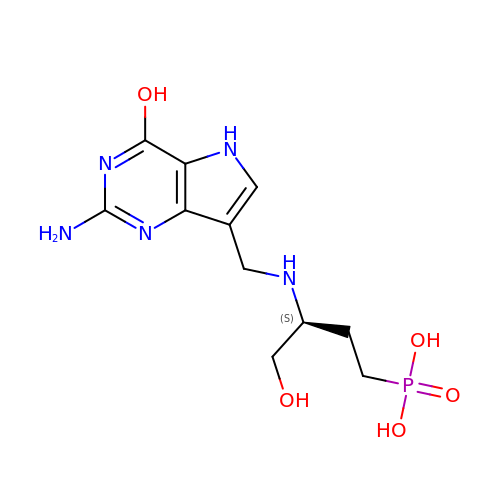[(3S)-3-{[(2-amino-4-hydroxy-5H-pyrrolo[3,2-d]pyrimidin-7-yl)methyl]amino}-4-hydroxybutyl]phosphonic acid | C11 H18 N5 O5 P | WDBHHLGLZFXXDD-ZETCQYMHSA-N ERDRP-0519 is a potent nonnucleoside inhibitor active against measles virus (MeV) and other Morbilliviruses. Conversely, polymerase inhibitors like ERDRP-0519 show greater promise due to the high conservation of the L-P complex across MeV strains. Here we report cryo-EM structures of the compound bound to MeV polymerase complexes at 2.73 Å and 2.48 Å resolution, revealing a unique binding pocket in the RdRp palm subdomain that overlaps the catalytic GDN motif. Structural analysis revealed that ERDRP-0519 binds to the palm subdomain of the RdRp, targeting the catalytic GDN motif and a nearby hydrophobic channel.

To test this, we assembled the MeV ternary polymerase complex14 with ERDRP-0519 and analyzed it by cryo-EM. The maps revealed two complexes: Lcore-P and Lfull-P-C, with clear ERDRP-0519 density on the L protein. Additionally, C protein presence did not alter the binding mode, suggesting stable drug association across RNA synthesis states. First, it inhibits the catalytic center by interacting with residue D773 in the GDN motif. The piperidine group displaces D773, creating space for hydrophobic interaction that directly impairs active site function. Second, although the morpholine ring does not directly contact the L protein, structural comparison with the NiV L-P-RNA complex17 shows steric clashes, suggesting the morpholine ring obstructs RNA binding. A strong hydrogen bond (2.8 Å) forms between the compound’s carboxyl group in the linker and residue W671 of the L protein.

> MDSLSVNQILYPEVHLDSPIVTNKIVAILEYARVPHAYSLEDPTLCQNIKHRLKNGFSNQMIINNVEVGNVIKSKLRSYPAHSHIPYPNCNQDLFNIEDKESTRKIRELLKKGNSLYSKVSDKVFQCLRDTNSRLGLGSELREDIKEKVINLGVYMHSSQWFEPFLFWFTVKTEMRSVIKSQTHTCHRRRHTPVFFTGSSVELLISRDLVAIISKESQHVYYLTFELVLMYCDVIEGRLMTETAMTIDARYTELLGRVRYMWKLIDGFFPALGNPTYQIVAMLEPLSLAYLQLRDITVELRGAFLNHCFTEIHDVLDQNGFSDEGTYHELIEALDYIFITDDIHLTGEIFSFFRSFGHPRLEAVTAAENVRKYMNQPKVIVYETLMKGHAIFCGIIINGYRDRHGGSWPPLTLPLHAADTIRNAQASGDGLTHEQCVDNWKSFAGVKFGCFMPLSLDSDLTMYLKDKALAALQREWDSVYPKEFLRYDPPKGTGSRRLVDVFLNDSSFDPYDVIMYVVSGAYLHDPEFNLSYSLKEKEIKETGRLFAKMTYKMRACQVIAENLISNGIGKYFKDNGMAKDEHDLTKALHTLAVSGVPKDLKESHRGGPVLKTYSRSPVHTSTRNVRAAKGFIGFPQVIRQDQDTDHPENMEAYETVSAFITTDLKKYCLNWRYETISLFAQRLNEIYGLPSFFQWLHKRLETSVLYVSDPHCPPDLDAHIPLYKVPNDQIFIKYPMGGIEGYCQKLWTISTIPYLYLAAYESGVRIASLVQGDNQTIAVTKRVPSTWPYNLKKREAARVTRDYFVILRQRLHDIGHHLKANETIVSSHFFVYSKGIYYDGLLVSQSLKSIARCVFWSETIVDETRAACSNIATTMAKSIERGYDRYLAYSLNVLKVIQQILISLGFTINSTMTRDVVIPLLTNNDLLIRMALLPAPIGGMNYLNMSRLFVRNIGDPVTSSIADLKRMILASLMPEETLHQVMTQQPGDSSFLDWASDPYSANLVCVQSITRLLKNITARFVLIHSPNPMLKGLFHDDSKEEDEGLAAFLMDRHIIVPRAAHEILDHSVTGARESIAGMLDTTKGLIRASMRKGGLTSRVITRLSNYDYEQFRAGMVLLTGRKRNVLIDKESCSVQLARALRSHMWARLARGRPIYGLEVPDVLESMRGHLIRRHETCVICECGSVNYGWFFVPSGCQLDDIDKETSSLRVPYIGSTTDERTDMKLAFVRAPSRSLRSAVRIATVYSWAYGDDDSSWNEAWLLARQRANVSLEELRVITPISTSTNLAHRLRDRSTQVKYSGTSLVRVARYTTISNDNLSFVISDKKVDTNFIYQQGMLLGLGVLETLFRLEKDTGSSNTVLHLHVETDCCVIPMIDHPRIPSSRKLELRAELCTNPLIYDNAPLIDRDATRLYTQSHRRHLVEFVTWSTPQLYHILAKSTALSMIDLVTKFEKDHMNEISALIGDDDINSFITEFLLIEPRLFTIYLGQCAAINWAFDVHYHRPSGKYQMGELLSSFLSRMSKGVFKVLVNALSHPKIYKKFWHCGIIEPIHGPSLDAQNLHTTVCNMVYTCYMTYLDLLLNEELEEFTFLLCESDEDVVPDRFDNIQAKHLCVLADLYCQPGTCPPIQGLRPVEKCAVLTDHIKAEAMLSPAGSSWNINPIIVDHYSCSLTYLRRGSIKQIRLRVDPGFIFDALAEVNVSQPKIGSNNISNMSIKAFRPPHDDVAKLLKDINTSKHNLPISGGNLANYEIHAFRRIGLNSSACYKAVEISTLIRRCLEPGEDGLFLGEGSGSMLITYKEILKLSKCFYNSGVSANSRSGQRELAPYPSEVGLVEHRMGVGNIVKVLFNGRPEVTWVGSVDCFNFIVSNIPTSSVGFIHSDIETLPDKDTIEKLEELAAILSMALLLGKIGSILVIKLMPFSGDFVQGFISYVGSHYREVNLVYPRYSNFISTESYLVMTDLKANRLMNPEKIKQQIIESSVRTSPGLIGHILSIKQLSCIQAIVGDAVSRGDINPTLKKLTPIEQVLINCGLAINGPKLCKELIHHDVASGQDGLLNSILILYRELARFKDNQRSQQGMFHAYPVLVSSRQRELISRITRKFWGHILLYSGNRKLINKFIQNLKSGYLILDLHQNIFVKNLSKSEKQIIMTGGLKREWVFKVTVKETKEWYKLVGYSALIKD;>[4x]MAEEQARHVKNGLECIRALKAEPIGSLAIEEAMAAWSEISDNPGQERATCREEKAGSSGLSKPCLSAIGSTEGGAPRIRGQGPGESDDDAETLGIPPRNLQASSTGLQCHYVYDHSGEAVKGIQDADSIMVQSGLDGDSTLSGGDNESENSDVDIGEPDTEGYAITDRGSAPISMGFRASDVETAEGGEIHELLRLQSRGNNFPKLGKTLNVPPPPDPGRASTSGTPIKKGTDARLASFGTEIASSLTGGATQCARKSPSEPSGPGAPAGNVPECVSNAALIQEWTPESGTTISPRSQNNEEGGDHYDDELFSDVQDIKTALAKIHEDNQKIISKLESLLLLKGEVESIKKQINRQNISISTLEGHLSSIMIAIPGLGKDPNDPTADVEINPDLKPIIGRDSGRALAEVLKKPVASRQLQGMTNGRTSSRGQLLKEFQLKPIGKKMSSAVGFVPDTGPASRSVIRSIIKSSRLEEDRKRYLMTLLDDIKGANDLAKFHQMLMKIIMKSG;>[2x]MSKTDWNASGLSRPSPSAHWPSRKLWQHGQKYQTTQDRSEPPAGKRRQAVRVSANHASQQLDQLKAVHLASAVRDLERAMTTLKLWESPQEISRHQALGYSVIMFMITAVKRLRESKMLTLSWFNQALMVIAPSQEETMNLKTAMWILANLIPRDMLSLTGDLLPSLWGSGLLMLKLQKEGRSTSS>[2x]IE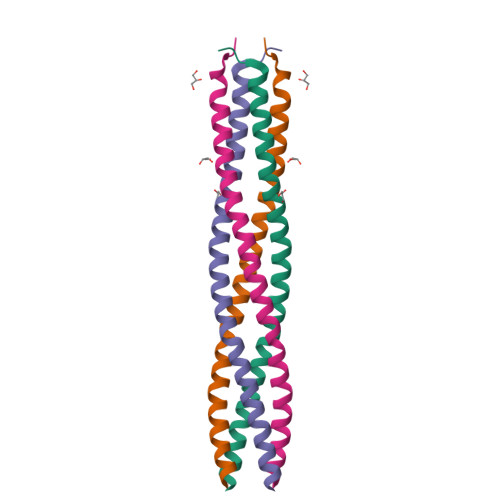GSTQSDGWEMKSRSLSGAIHPVLQSPLQQGDLNALVTSVQSLALNVNEILNTVRNLDSRMNQLETKVDRILSSQSLIQTIKNDIVGLKAGMATLEGMITTVKIMD>[2x]KHSLPDLPYDYGALEPHINAQIMQLHHSKNHAAYVNNLNVTEEKYQEALAKGDVTA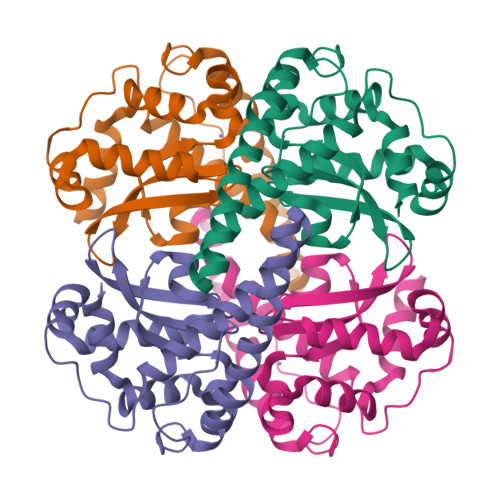QIALQPALKFNGGGHINHSIFWTNLSPNGGGEPKGELLEAIKRDFGSFDKFKEKLTAASVGVQGSGWGWLGFNKERGHLQIAACPNQDPLQGTTGLIPLLGIDVWEHAYFLQYKNVRPDYLKAIWNVINWENVTERYMACKK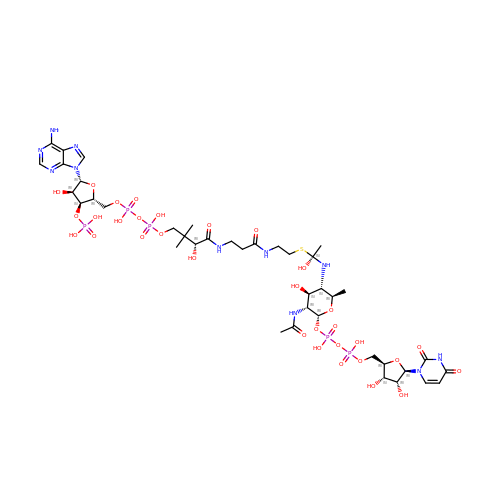[(2~{R},3~{R},4~{S},5~{S},6~{R})-3-acetamido-5-[[(1~{S})-1-[2-[3-[[(2~{R})-4-[[[(2~{R},3~{S},4~{R},5~{R})-5-(6-aminopurin-9-yl)-4-oxidanyl-3-phosphonooxy-oxolan-2-yl]methoxy-oxidanyl-phosphoryl]oxy-oxidanyl-phosphoryl]oxy-3,3-dimethyl-2-oxidanyl-butanoyl]amino]propanoylamino]ethylsulfanyl]-1-oxidanyl-ethyl]amino]-6-methyl-4-oxidanyl-oxan-2-yl] [[(2~{R},3~{S},4~{R},5~{R})-5-[2,4-bis(oxidanylidene)pyrimidin-1-yl]-3,4-bis(oxidanyl)oxolan-2-yl]methoxy-oxidanyl-phosphoryl] hydrogen phosphate | C40 H66 N11 O32 P5 S | CHRNLGHDEXUXFL-IOFFXKHASA-N>MQGVN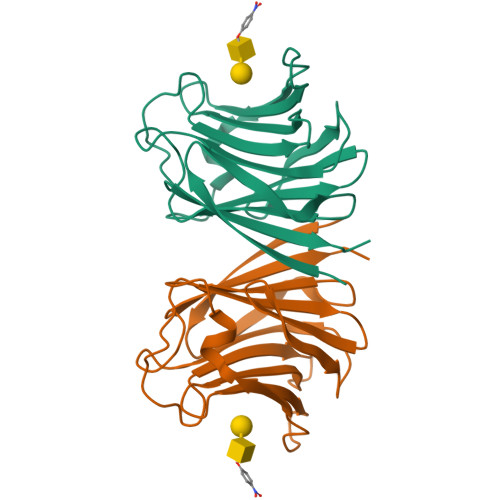IYNISAGTSVDLAAPVTTGDIVTFFSSALNLNAGAGNPNNTTLNLFAENGAYLLHIAFRLQANVIIFNSRQPDGPWLVEQRVSDVANQFAGIDGKAMVTVFDHGDKYQVVINEKTVIQYTKQISGLTSSLSYNATEETSIFSTVVEAVTYTGLALE[4x]6-bromo-2-[1-methyl-3-(propan-2-yl)-1H-pyrazol-4-yl]-1H-imidazo[4,5-b]pyridine | C13 H14 Br N5 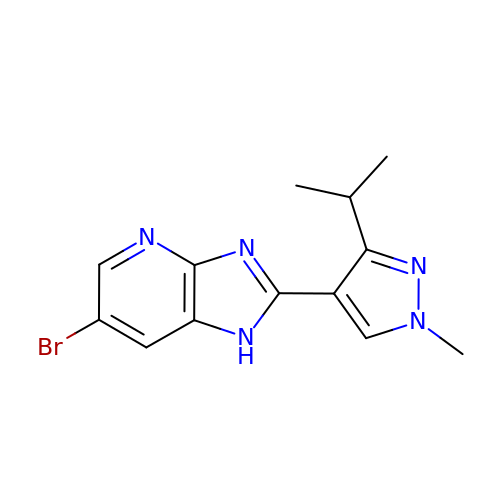| XYHWYOLLASBNRO-UHFFFAOYSA-N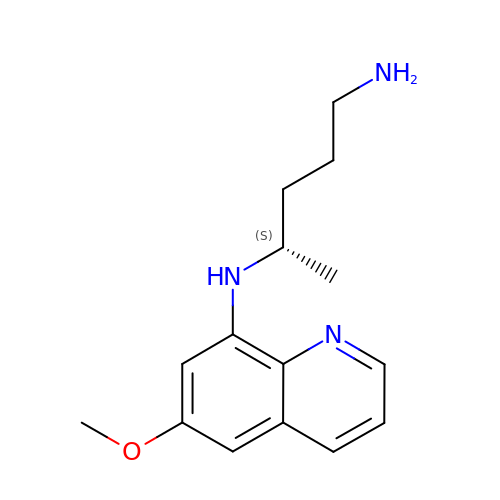(4S)-N~4~-(6-methoxyquinolin-8-yl)pentane-1,4-diamine | C15 H21 N3 O | INDBQLZJXZLFIT-NSHDSACASA-N2-[3-[(1~{R})-1-[(2~{S})-1-[(2~{S})-2-(5-chloranylthiophen-2-yl)propanoyl]piperidin-2-yl]carbonyloxy-3-(3,4-dimethoxyphenyl)propyl]phenoxy]ethanoic 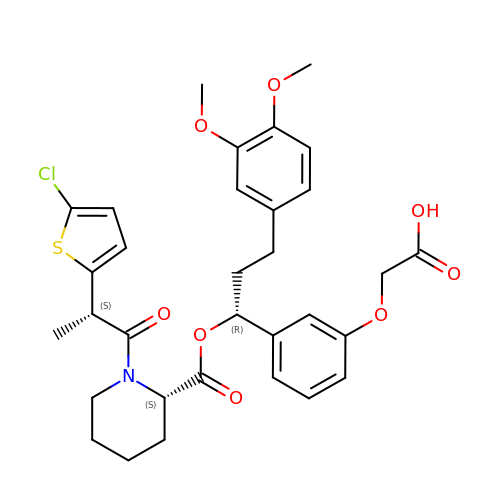acid | C32 H36 Cl N O8 S | OIYSSIJKGXDGIE-DCEDVJGZSA-N> MSNTYSISVETGGYRQLDLFAERCGEGNAVVTVADGNGVAIAAHTMPIAERRHHFSIAVPQKSTVTVAASGLVVRFGYLSECDDLLDNGVRYVNMNPSDTDWPAQPTLEQIYNRFGRSGAHFEPFARWMNDPNGLCQFQGRYHLFFQLNPYGFGWDNMHWGHAVSRDLVHWTHLPVFLEPQPELHTDERIVGGAFSGSAVTVDEHDNPVAGNEANAIRLYLTRHLETRGDESSVTEYQTTCLCEDGVHVRVESPVALRANDDFGYDFRDPKVECGMGGEALDPDRAYMVTATNLPVSEFGADAADSAVPGISTQNTGGWFTYSPQGKPGVDQPNNATVPAMTLFSAKKPLK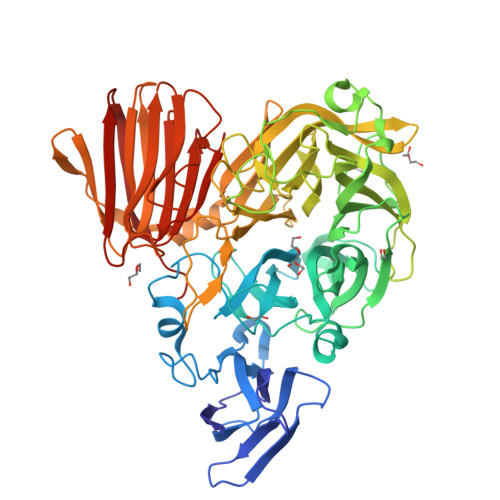RNVTWRYEGPVLADFGHQIARTYECPDLFQVDGVTVAVGALMHYRDKQGRFQQVRWYAGDLVNTDNGPKLDVKASDWCDFGTGYYATQSFADDNGRRIVFGWFTDFPEMRVEQPCLANGMMSLPRELHVRDGRLYSKPVSEVYRELLGERLAVHGDGGDMVVTAPGNAYYANVHLADDADAIMVLAKGVNPQDGRPTELLLQRTDGVTRLVAKGTAVEDVDFDSGITDVRQVEVFFDRNVVEVFLNGGQTAGSMLFQGADGDGELRIASSGKIDAVDARALNGIWR>MLNQFPGQYSNNIFCFPPIESETKSGKKASWIICVQVVQHNTIIPITDEMFSTDVKDAVAEIFTKFFVEEGAVRISKMTRVTEGKNLGKKNATTVVHQAFKDALSKYNRHARQKRGAHTNRGMIPPMLVKYFNIIPKTFFEEETDPIVQRKRNGVRAVACQQGDGCILLYSRTEKEFLGLDNIKKELKQLYLFIDVRVYLDGELYLHRKPLQWIAGQANAKTDSSELHFYVFDCFWSDQLQMPSNKRQQLLTNIFKQKEDLTFIHQVENFSVKNVDEALRLKAQFIKEGYEGAIVRNANGPY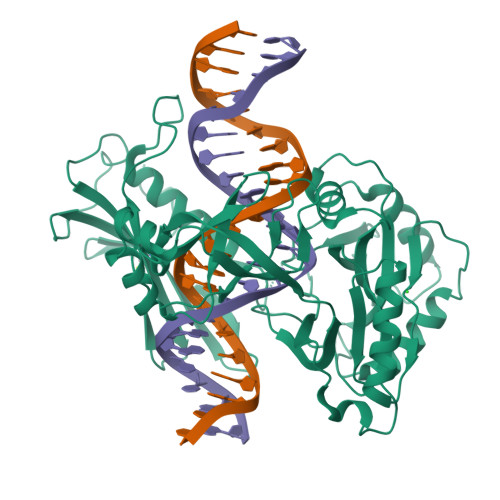EPGYNNYHSAHLAKLKPLLDAEFILVDYTQGKKGKDLGAILWVCELPNKKRFVVTPKHLTYADRYALFQKLTPALFKKHLYGKELTVEYAELSPKTGIPLQARAVGFREPINVLEII[2x]3-(benzyloxy)-N-(4-methyl-1,3-thiazol-2-yl)pyridin-2-amine 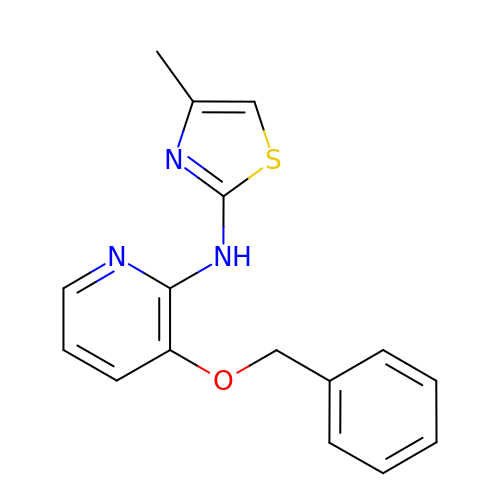| C16 H15 N3 O S | LPJWCRSWBACCSH-UHFFFAOYSA-N> GELELQRQKRSINLQQPRMATERGNLVFLTGSAQNIEFRTGSLGKIKLNDEDLSECLHQIQKNKEDIIELKGSAIGLPQ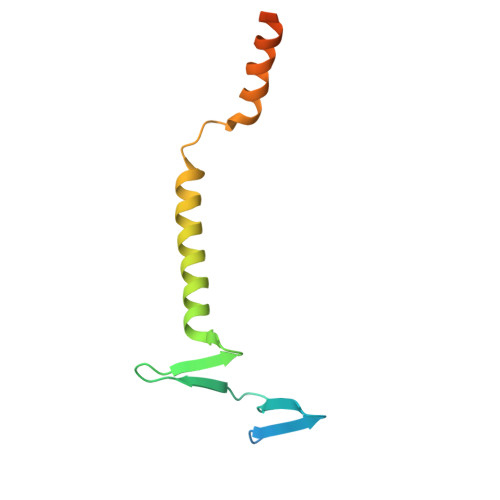NISSQIYQLNSKLVDLERKFQGLQQTVDKKV>[2x]GSHMVKDTLFSTPIAKLGDFIFDENVAEVFPDMIQRSVPGYSNIITAIGMLAERFVTADSNVYDLGCSRGAATLSAR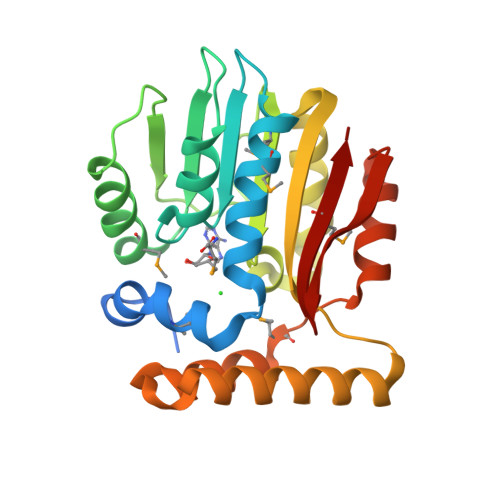RNINQPNVKIIGIDNSQPMVERCRQHIAAYHSEIPVEILCNDIRHVEIKNASMVILNFTLQFLPPEDRIALLTKIYEGLNPNGVLVLSEKFRFEDTKINHLLIDLHHQFKRANGYSELEVSQKRTALENVMRTDSIETHKVRLKNVGFSQVELWFQCFNFGSMIAVK>[2x]GSHMSVDLDPSARFAEYAHPERLVSTEWLAAHLGDEGLVVVESDEDVLLYETGHIPGAVKVDWHTDLNDPVQRDYIDGAAFAALLGERGISRDTTVVIYGDKNNWWAAYALWVFTLFGHDDVRLLDGGRSKWEAEGRAY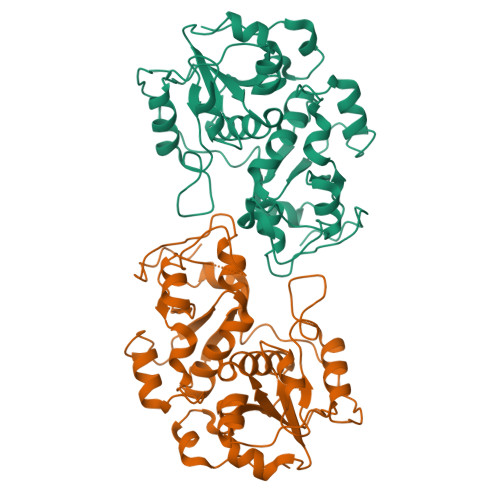TTDAPTVAATSYPVVERDDSRIRAYRDDVLAHFGKPLIDVRSPEEFSGARTTAPAYPEEGALRAGHIPSAQNVPWGKAAAEDGTFRTLAELDALYRDGAGLKDGDDVVAYCRIGERSSHTWFVLQHLLGFENVRNYDGSWTEWGSAVRVPIVQGSEPGEAPAPIVGR> DPGCRLRSQLVPVRALGLGHRSDELVRFRFCSGSCRRARSPHDLSLASLLGAGALRPPPGSRPVSQPC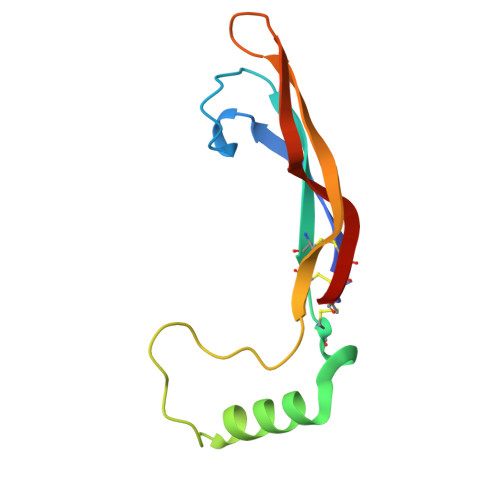CRPTRYEAVSFMDVNSTWRTVDRLSATACGCLG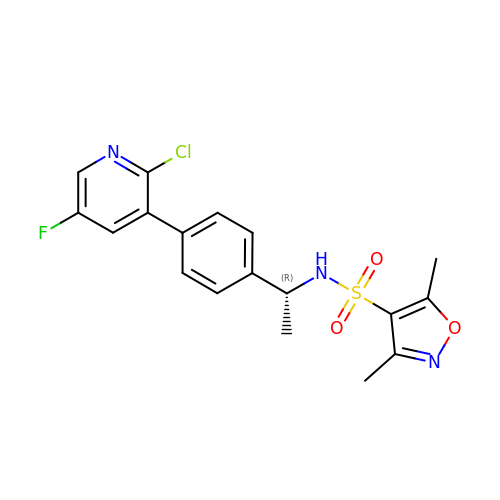N-{(1R)-1-[4-(2-CHLORO-5-FLUOROPYRIDIN-3-YL)PHENYL]ETHYL}-3,5-DIMETHYLISOXAZOLE-4-SULFONAMIDE | C18 H17 Cl F N3 O3 S | UOZIRTCHSJAAOG-SNVBAGLBSA-N(~{E})-3-[3-(2-methyl-5-phenyl-phenyl)-4-oxidanyl-phenyl]prop-2-enoic 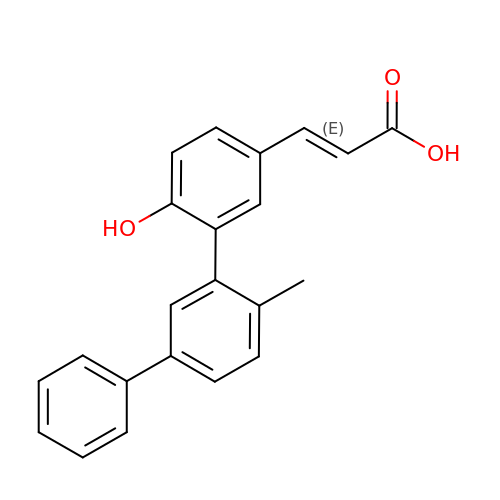acid | C22 H18 O3 | ZVBMBUNLXBSQPU-FMIVXFBMSA-N>[2x]MGLMNAFDSQTEDSSPAIGRNLRSRPLARKKLSEMVEEELEQMIRRREFGEGEQLPSERELMAFFNVGRPSVREALAALKRKGLVQINNGERARVSRPSADTIIGELSGMAKDFLSHPGGIAHFEQLRLFFESSLVRYAAEHATDEQIDLLAKALEINSQSLDNNAAFIRSDVDFHRVLAEIPGNPIFMAIHVALLDWLIAARPTV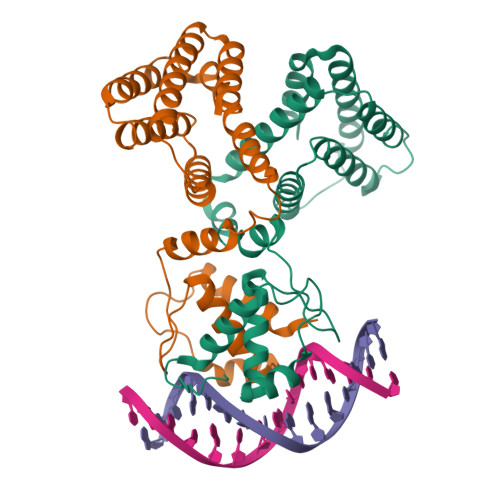TDQALHEHNNVSYQQHIAIVDAIRRHDPDEADRALQSHLNSVSATWHAFGQTTNKKK> MIPQTLTNTNLFIDGVSFAGDVPSLTLPKLAVKTEQYRAGGMDAPVSIDMGLEA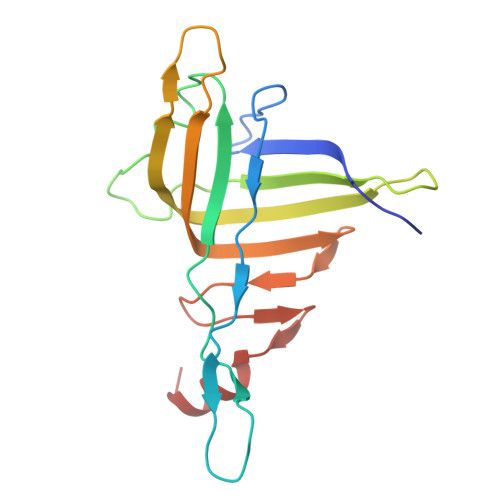MEAKFSTNGARREALNFFGLADQSAFNGVFRGSFKGQKGASVPVVATLRGLLKEVDPGDWKAGEKAEFKYAVAVSYYKLEVDGREVYEIDPVNGVRAINGVDQLAGMRNDLGL>[2x]MRVLLIAGGVSPEHEVSLLSAEGVLRHIPFPTDLAVIAQDGRWLLGEKALTALEAKAAPEGEHPFPPPLSWERYDVVFPLLHGRFGEDGTVQGFLELLGKPYVGAGVAASALCMDKDLSKRVLAQAGVPVVPWVAVRKGEPPVVPFDPPFFVKPANTGSSVGIS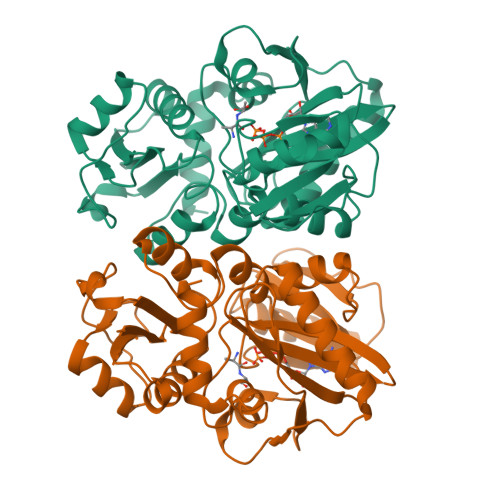RVERFQDLEAALALAFRYDEKAVVEKALSPVRELEVGVLGNVFGEASPVGEVRYEAPFYDYETKYTPGRAELLIPAPLDPGTQETVQELALKAYKVLGVRGMARVDFFLAEGELYLNELNTIPGFTPTSMYPRLFEAGGVAYPELLRRLVELALT>XTPRQARAARAAAC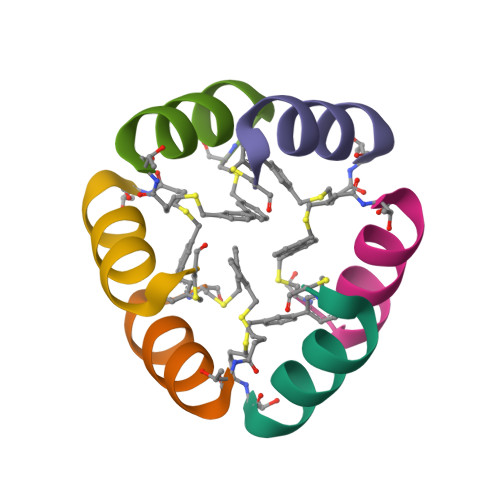X[6x]> MSLKNSSRSAVDPFIVMDVMEAARRAEEAGRRIIHMEVGQPGTGAPRGAVEALAKSLETDALGYTVALGLPALRQRIARLYGEWYGVDLDPGRVVITPGSSGGFLLAFTALFDSGDRVGIGAPGYPSYRQILRALGLVPVDLPT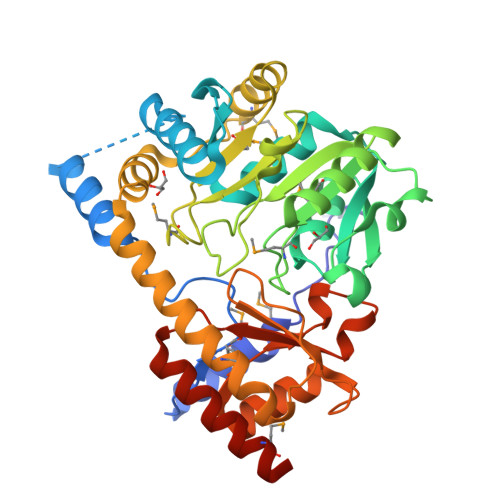APENRLQPVPADFAGLDLAGLMVASPANPTGTMLDHAAMGALIEAAQAQGASFISDEIYHGIEYEAKAVTALELTDECYVINSFSKYFSMTGWRVGWMVVPEDQVRVVERIAQNMFICAPHASQVAALAALDCDAELQANLDVYKANRKLMLERLPKAGFTRIAPPDGAFYVYADVSDLTDDSRAFAAEILEKAGVAVTPGLDFDPERGAGTLRFSYARATADIEEGLDRLEAFMQARGEGHHHHHH> SSQIRQNYSTEVEAAVNRLVNLYLRASYTYLSLGFYFDRDDVALCGVCHFFHELAEEKREGAERLLKMQNQRGGRALFQDLQKPSQDEWGTTLDAMKAAIVLEK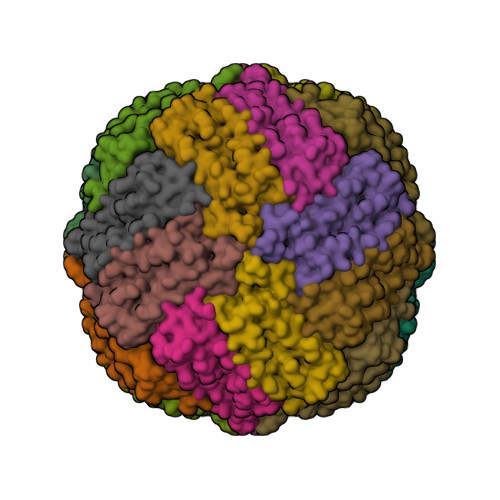SLNQALLDLHALGSAQADPHLCDFLESHFLDEEVKLIKKMGDHLTNIQRLVGSQAGLGEYLFERLTLKHD> MKIEEVKSTTKTQRIASHSHVKGLGLDESGLAKQAASGLVGQENAREACGVIVELIKSKKM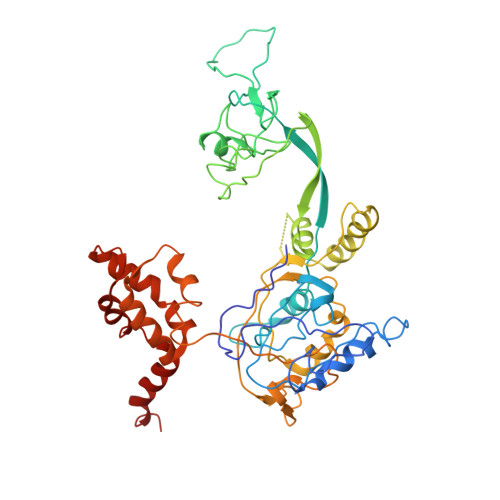AGRAVLLAGPPGTGKTALALAIAQELGSKVPFCPMVGSEVYSTEIKKTEVLMENFRRAIGLRIKETKEVYEGEVTELTPCETENPMGGYGKTISHVIIGLKTAKGTKQLKLDPSIFESLQKERVEAGDVIYIEANSGAVKRQGRCDTYATEFDLEAEEYVPLPKGDVHKKKEIIQDVTLHDLDVANARPQGGQDILSMMGQLMKPKKTEITDKLRGEINKVVNKYIDQGIAELVPGVLFVDEVHMLDIECFTYLHRALESSIAPIVIFASNRGNCVIRGTEDITSPHGIPLDLLDRVMIIRTMLYTPQEMKQIIKIRAQTEGINISEEALNHLGEIGTKTTLRYSVQLLTPANLLAKINGKDSIEKEHVEEISELFYDAKSSAKILADQQDKYMK> MGSSHHHHHHSQDPMSRQANRGTESKKMSSELFTLTYGALVTQLCKDYENDEDVNKQLDKMGFNIGV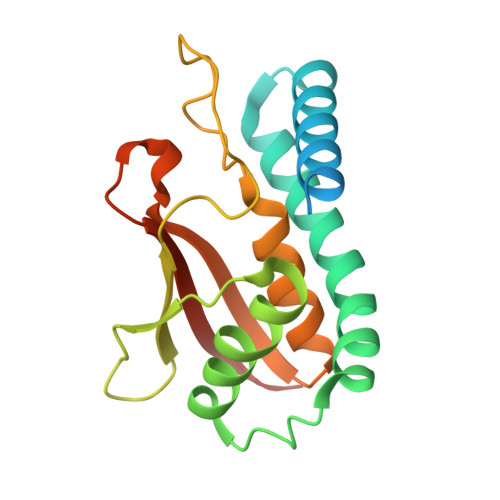RLIEDFLARSNVGRAHDFRETADVIAKVAFKMYLGITPSITNWSPAGDEFSLILENNPLVDFVELPDNHSSLIYSNLLCGVLRGALEMVQMAVEAKFVQDTLKGDGVTEIRMRFIRRIEDNLPAGEE> MDFLDFEKVFSFYSKATKKGFSPFFVPALEKAEEPAGNFFLDRKGNLFSIREDFTKTVLNHRKRYSPESQIKVWYADFVYRYSGSDLVAEYQLGLEKVPRNSLDDSLEVLEIIVESASEFFEGP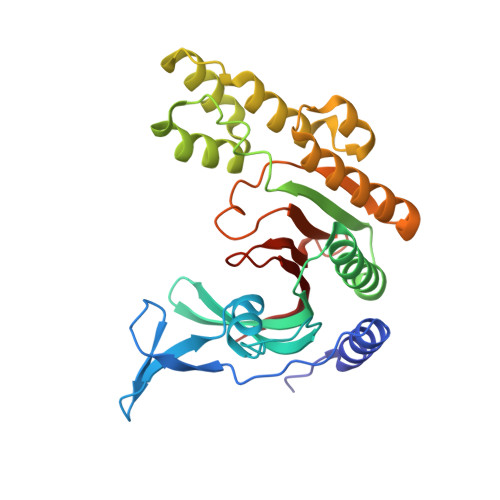VIVEIGHTGLYEDLLKEIPKDLHEKVLNLIDTKNLAEIEFLSHMKKIDLSRVEKIIEDSIYRRSPEHLKTMDLPLSVREDLLSASSFLQEKFPTVSVEIDLTLARTIEEYCGLIFTIYDTSSSRLVAAGGEYTVNGEKGVGGSIFLEGKTC> MHHHHHHHHHHGENLYFQGMEGKKYTIGTDLTFAPFEFQDSKGKYIGIDVDLLDAIAKDQDFEVDLKPLGFDSAVQAIQSKQIDGMIAGMSITDERKKSFDFSDPY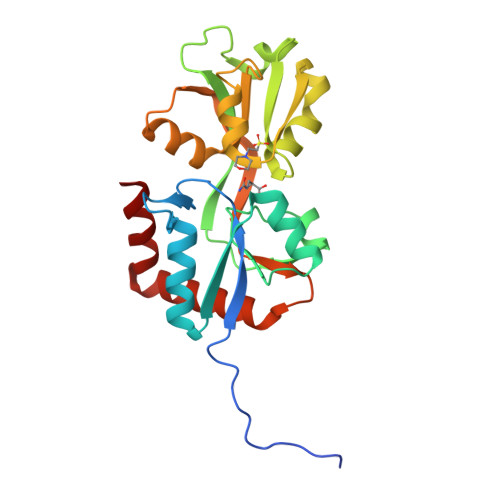FDSGLQLAVKKGNDKIKSYDDLKGKTVAAKVGTESANFLEKNKEKYDYTIKNFDDATGLYKALENGEADAIVDDYPVLGYAVKNGQKLQLVGDKETGSSYGFAVKKGQNPELIKKFNAGLKNLKDNGTYDKILNNYLA> MKRVFVFQDFKSQKFWSIDVRGTDVIVNYGKLGTDGQTQVKNFSSAGEAEKAAGKLIAEKTKKGYVETLEEVAKEMKVEAKKYALSYDEAEEGVNLMDKILKDKKLPSLKQITIGCWGYEGEDCSDIADGIVENKEKFAHFEGLFWGDIDFEEQEISWIEQVDLSPVLD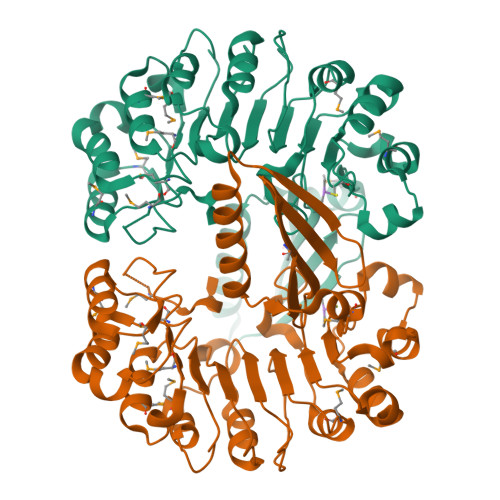AMPLLNNLKIKGTNNLSIGKKPRPNLKSLEIISGGLPDSVVEDILGSDLPNLEKLVLYVGVEDYGFDGDMNVFRPLFSKDRFPNLKWLGIVDAEEQNVVVEMFLESDILPQLETMDISAGVLTDEGARLLLDHVDKIKHLKFINMKYNYLSDEMKKELQKSLPMKIDVSDSQEYDDDYSYPMITELEHHHHHH> GPLGSPLTASMLASAPPQEQKQMLGERLFPLIQAMHPTLAGKITGMLLEIDNSELLHMLESPESLRSKVDEAVAVLQAHQAKEAAQKA;> RQLNVNAKPFVPNVH

Cytoplasmic poly(A)-binding protein (PABP), also termed PABPC or PABPC1, is an essential protein that binds to and mediates the stimulatory effect of the poly(A) tail on translation initiation. Previous studies showed that MLLE is a peptide-binding domain that specifically recognizes a conserved PAM2 (for PABP-interacting motif 2) sequence. Unlike other PAM2-containing proteins, eRF3 possesses two overlapping PAM2 sequences (PAM2-N and PAM2-C), which each independently bind to the MLLE domain of PABPC1 with low micromolar affinity. Here, we determined two crystal structures of the MLLE domain of human PABPC1 in complex with the PAM2-N and PAM2-C peptides from human eRF3.

We obtained well-diffracting co-crystals with eRF3 residues 67–81 (PAM2-N) and 76–90 (PAM2-C). Overlay of the MLLE/PAM2-N and MLLE/PAM2-C structures reveals striking similarity of the bound conformations despite the highly divergent peptide sequences. In both structures, the peptide binds by wrapping around the highly conserved KITGMLLE signature motif of MLLE and interacting with the hydrophobic pockets between helices α2 and α3 and between helices α3 and α5 of MLLE. The peptides adopt an extended conformation interrupted by a β-turn at residues Asn70-Val71-Asn72 in PAM2-N and at residues Asn79-Val80-His81 in PAM2-C. In the N-terminal part of the peptide, the side chain of eRF3 Leu69 of PAM2-N inserts into a hydrophobic pocket formed by the side chains of Met584, Ile588, Ala610 and the aliphatic parts of Lys606 and Glu609. At the tip of the peptide β-turn, the side chain of Val71/Val80 makes an additional hydrophobic contact with the MLLE side chains of Val613 and His617. Another hydrophobic interaction involves the invariantly conserved alanine at residue 73 of PAM2-N and at 82 of PAM2-C. At the C-terminus of both peptides, Phe76/Phe85 fits into the shallow cavity formed by Gly563, the methyl groups of Thr582 and Leu586 and the aliphatic part of Glu564. In addition to its essential side chain, the amide of Phe76/Phe85 hydrogen bonds with the carbonyl of Gly579. Thus eRF3 Phe76 plays two distinct roles in the complexes, alternately occupying the hydrophobic pocket between MLLE helices α2 and α3 in the PAM2-N complex and between helices α3 and α5 in the PAM2-C complex. The simultaneous requirement for Phe76 for MLLE binding by both PAM2-N and PAM2-C explains the previous observations of a one-to-one stoichiometry of eRF3 binding to PABPC1 despite the existence of two PAM2 motifs.> GSTTENEKSRSLPAERNPLYKDDTLDHTPLIPKCRAQVIEFPDGPATFVRLKCTNPESKVPHFLMRMAKDSSISATSMFRSAFPKATQEEEDLEMRWIRDNLNPIEDKRVAGLWV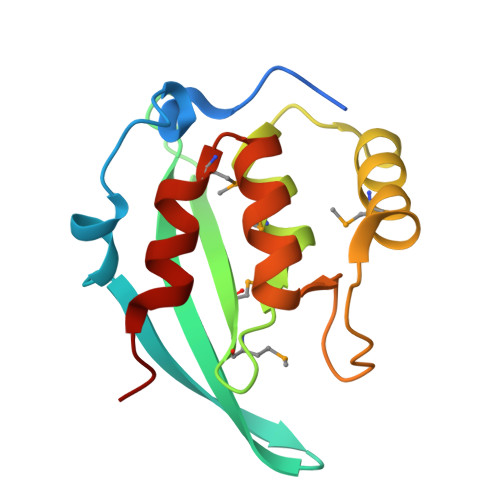PPADALALAKDYSMTPFINALLEASST> MADAAVIEKLEAGFKKLEAATDCKSLLKKYLTKEVFDKLKDKRTSLGATLLDVIQSGVENLDSGVGIYAPDAEAYTLFAPLFDPIIEDYHVGFKQTDKHPNKDFGDVNSFVNVDPEGKFVISTRVRCGRSMQGYPFN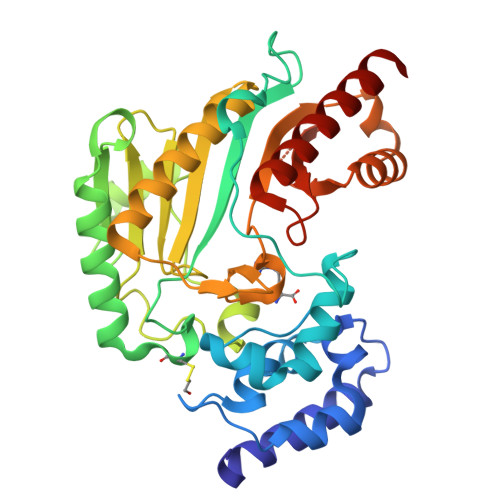PCLTESQYKEMEAKVSSTLSSLEGELKGTYYPLTGMSKEVQQKLIDDHFLFKEGDRFLQAANACRYWPAGRGIYHNDNKTFLVWVNEEDHLRIISMQMGGDLGQVFRRLTSAVNEIEKRIPFSHHDRLGFLTFCPTNLGTTVRASVHIKLPKLAANEEKLEEVAGKYNLQVRGTRGEHTEAEGGIYDISNKRRMGLTEFQAVKEMEDGILELIKIEKEM BETA-D-GLUCOPYRANOSE 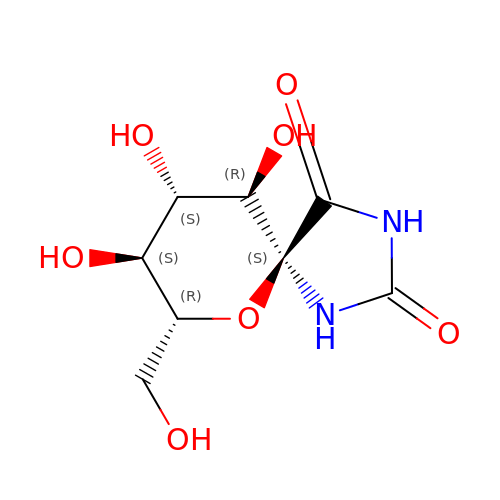SPIROHYDANTOIN | C8 H12 N2 O7 | QRXBDPYWCAAAAI-WWHASAIZSA-N> MKSSHHHHHHENLYFQSNAEESAQQRSERYVSARSQHPAWLLLASRRAPLVLGCLRTLFERAHDGIPMEDALQALSEMLAAYASQELYEIDPDATHLQAGRELREWIKRRLVVEREGRIYATDALESAIQFVDSLDSRIMTSTASRLSVVQREIENLETGLNPSPTGRIASLRRRIQDLEHELARVEAGHVDVLDEAQAIEGMREVYNLATSLRADFRRVEDSWREADRALRHSIISEQSHRGEIVDRLLDGQDALLNTP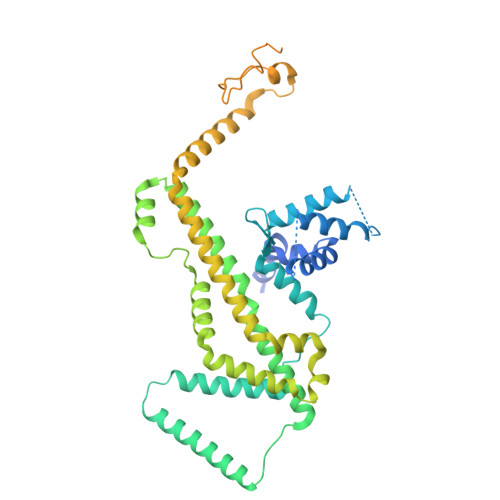EGRVFESFQQQLRQSAELEVMRERLRTILRHPAVPKALNRPQQRELRWLALRLVRESQAVLQARARSERDVRGFMKTGLAAEHHRVGQLLNDFFNLALSVDWQRQSERRKPACLPPVGVAITGVPAIERLRFKTLDDDDAGELDLSLKPAGLEQIDDDFWDAFDGLDREALIHDTLAVLVEQGRPVSLGELASLLPPAHDLETFALWLAMAREAGIEVLTEERQFVELVDEDEQRWGFNLPYVGLDHEALKDIDWEL> AMDMYVVIVYDVAVERVNRVKKFLRRHLHWVQNSVFEGEVTLAEFERIKAGLLDLIDEDEDSVVIYKLRSMPKREVLGMEKNP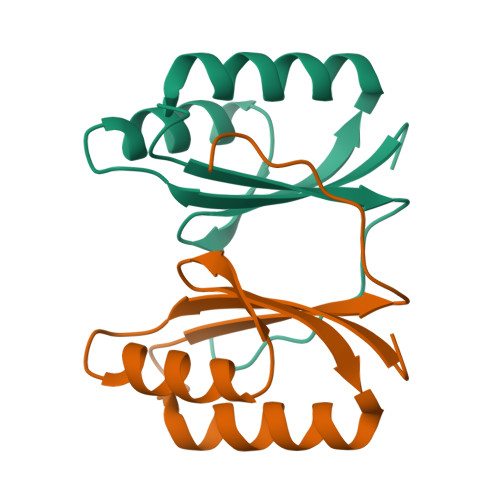LEDII>MRRRSRMLLCFAFLWVLGIAYYMYSGGGSALAGGAGGGAGRKEDWNEIDPIKKKDLHHSNGEEKAQSMETLPPGKVRWPDFNQEAYVGGTMVRSGQDPYARNKFNQVESDKLRMDRAIPDTRHDQCQRKQWRVDLPATSVVITFHNEARSALLRTVVSVLKKSPPHLIKEIILVDDYSNDPEDGALLGKIEKVRVLRNDRREGLMRSRVRGADAAQAKVLTFLDSHCECNEHWLEPLLERVAEDRTRVVSPIADVINMDNFQYVGASADLKGGFDWNLVFKWDYMTPEQRRSRQGNPVAPIKTPMIAGGAFVMDKFYFEELGKYDMMMDVWGGENLEISFRVWQCGGSLEIIPCSRVGHVFRKQHPYTFPGGSGTVFARNTRRAAEVWMDEYKNFYYAAVPSARNVPYGNIQSRLELRKKLSCKPFKWYLENVYPELRVPDHQDIAFGALQQGTNCLDTLGHFADGVVGVYECHNAGGNQEWALTKEKSVKHMDLCLTVVDRAPGSLIKLQGCRENDSRQKWEQIEGNSKLRHVGSNLCLDSRTAKSGGLSVEVCGPALSQQWKFTLNLQQ[6x]

One of the largest GT families in the human genome is the polypeptide N-acetylgalactosaminyl (GalNAc) transferase family (GalNAc-T1…T20, abbreviated T1…T20). Transferring GalNAc to Ser/Thr side chains, GalNAc-Ts initiate abundant O-linked glycosylation in the secretory pathway (Bennett et al., 2012, Hang and Bertozzi, 2005). All GalNAc-Ts are type II transmembrane proteins with luminal GT and lectin domains connected through a flexible linker (Bennett et al., 2012, Hang and Bertozzi, 2005, Ten Hagen et al., 2003). We made use of the fact that a double mutation (“BH,” I253A/L310A double mutant in GalNAc-T2) re-programmed GalNAc-Ts to accept alkyne-containing uridine diphosphate (UDP)-GalNAc analogs such as compounds 1–4 instead of the native substrate UDP-GalNAc (Choi et al., 2019).

A co-crystal structure of BH-T2, Mn2+, and UDP-GalNAc analog 1 at 3.1-Å resolution helped us visualize how the BH-T2 active site mutations affect enzyme-substrate binding. BH-T2 indeed contains a hole that accommodates the alkyne side chain bump in UDP-GalNAc analog 1. The formation of additional van der Waals interactions between the enzyme and substrate explain why the KM of BH-T2 toward 1 (2.6 μM) is approximately 10-fold lower than the KM of WT-T2 toward UDP-GalNAc (30 μM) (Choi et al., 2019). In turn, the fact that the kcat of BH-T2/1 (0.158 s−1) is approximately 5-fold lower than the kcat of WT-T2/UDP-GalNAc (0.813 s−1) indicates that these additional interactions may slightly slow the ring distortion that is needed to mediate the nucleophilic attack (Lira-Navarrete et al., 2014). Compounds 1, 2, and 3 were specific substrates for BH- but not WT-GalNAc-Ts.>[2x]MGSHHHHHHDITSLYKKAGSAAAVLEENLYFQGSFTMRLKELGEFGLIDLIKKTLESKVIGDDTAPVEYCSKKLLLTTDVLNEGVHFLRSYIPE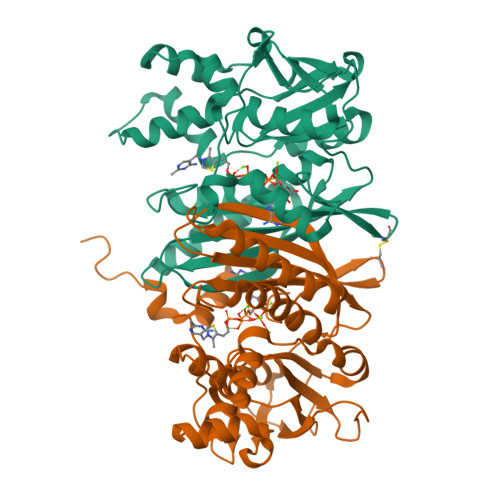AVGWKAISVNVSDVIANGGLPKWALISLNLPEDLEVSYVERFYIGVKRACEFYKCEVVGGNISKSEKIGISVFLVGETERFVGRDGARLGDSVFVSGTLGDSRAGLELLLMEKEEYEPFELALIQRHLRPTARIDYVKHIQKYANASMDISDGLVADANHLAQRSGVKIEILSEKLPLSNELKMYCEKYGKNPIEYALFGGEDYQLLFTHPKERWNPFLDMTEIGRVEEGEGVFVDGKKVEPKGWKHF> MLYTRRLMTTGGSATADGAVSYSKGSYHIVPKKYTVGKRIAVRSYLDRNRTELSDRTYMPQKAWFEPYTPKKFDMEHQRISHNFYNLETKLIWTAFDTPELIGILLHDETIKGAPHLYDAEFLESAVHWTRESRYWRCIGITKPFYNKTTLRAQCWHDRGLQVGTLVFSQAMRDALMDLERAVRRKELGLEPNYVWDRWGPVGFIDGARTDHLPRFAHNPYVDPDGVEVTEVDIAPFNTHEQIKERYGAFIDPDLRPFEGVFRAPSHGALTLDDVPHQEAVRLYRDLMEKADMPVMLGNG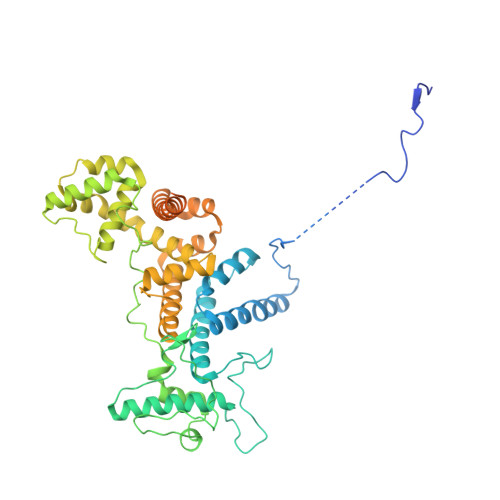AEIPPMDMRALFHLSANPERMKAASELSSWREVRGMLAPVQEVCDEKVEALRLMENTRHDAARVRTFYEEKCGFSDFMRTPDKVITAAVLCYLQELQRICTETDWGKPLARCLTDLERVNVMGKDAFLVYRHIEDAILDKKRRVWATRFAGEANEESTLDYLLENFGRRTEQTRNVGTTGTEFDREQEPIGRQVQRRVLDSDKASKLAEVRQKRGKMWSNKKSVFDSLHQKQLQNVTYGVH>[2x]MPAKVMRIGTMIKQLLEEVRAAPLDEASRNRLRDIHATSIRELEDGL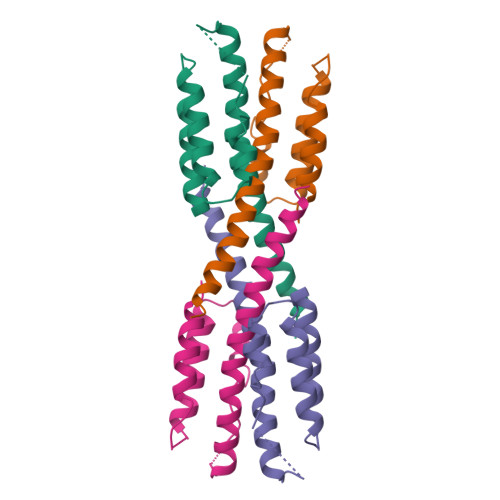APELREELDRLTLPFNEDAVPSDAELRIAQAQLVGWLEGLFHGIQTALFAQQMAARAQLQQMRQAALEHHHHHH> SSVGRSRSPPPSRERSVRSIEQELEQLRDVTPINQWKRKRSLWDIKPPGY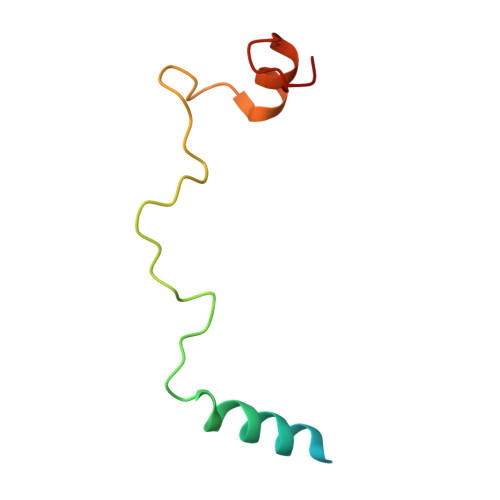ELVTADQAKMSGVFPLPGA>[2x]SGSMGHCRL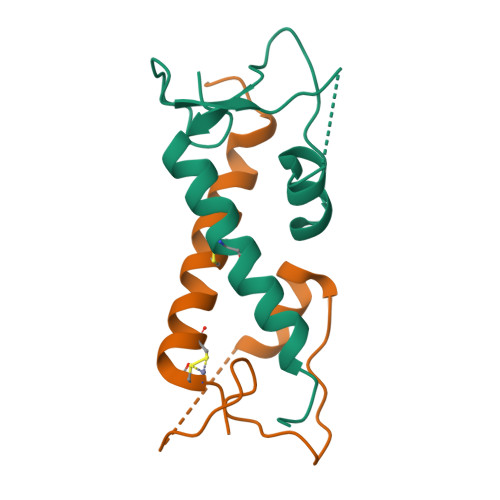CHGKFSSRSLRSISDRASGDSAERPFPGERVFVRDFQRLLGVAVHQDPALSQFVCRNCHAQFYQCHSLLESFLQRVNVSPM>[2x]CUUGCUGA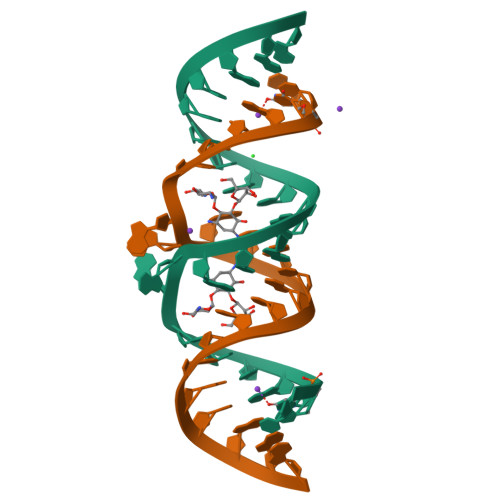AGUGCACACAGCAAG2-TERT-BUTYL-9-FLUORO-3,6-DIHYDRO-7H-BENZ[H]-IMIDAZ[4,5-F]ISOQUINOLINE-7-ONE | C18 H16 F N3 O | 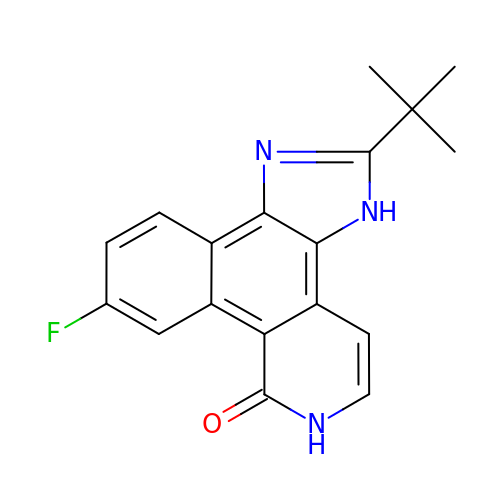VNDWQCSOSCCWIP-UHFFFAOYSA-N>RFLKVKNWETDVVLTDTLHLKSTLETGCTEHICMGSIMNPSQHTRKPEDVRTKDQLFPLAKEFLDQYYSSIKRFGSKAHMDRLEEVNKEIESTSTYQLKDTELIYGAKHAWRNASRCVGRIQWSKLQVFDARDCTTAHGMFNYICNHVKYATNKGNLRSAITIFPQRTDGKHDFRVWNSQLIRYAGYKQPDGSTLGDPANVQFTEICIQQGWKAPRGRFDVLPLLLQANGNDPELFQIPPELVLEVPIRHPKFDWFKDLGLKWYGLPAVSNMLLEIGGLEFSACPFSGWYMGTEIGVRDYCDNSRYNILEE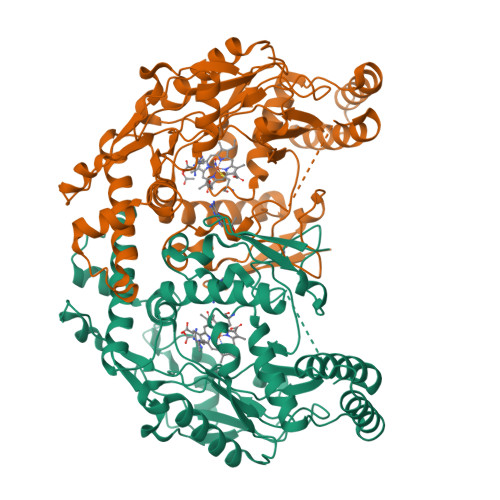VAKKMDLDMRKTSSLWKDQALVEINIAVLYSFQSDKVTIVDHHSATESFIKHMENEYRCRGGCPADWVWIVPPMSGSITPVFHQEMLNYRLTPSFEYQPDPWNTHVWKG[2x]>MSEKYIVTWDMLQIHARKLASRLMPSEQWKGI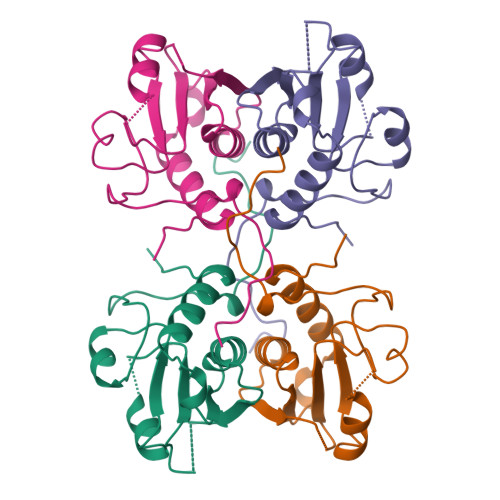IAVSRGGLVPGALLARELGIRHVDTVAISSYDHDNQRELKVLKRAEGDGEGFIVIDDLVDTGGTAVAIREMYPKAHFVTIFAKPAGRPLVDDYVVDIPQDTWIEQPWDMGVVFVPPISGR[2x]In bacteria, two distinct G3P acyltransferases (GPATs), PlsB and PlsY, catalyse the committed step. By contrast, the recently identified membrane-integral PlsY exists exclusively and ubiquitously in bacteria, and uses an unusual acyl donor, namely the acyl-phosphate (acylP), representing a unique class of acyltransferase. PlsY acylates G3P using acylP, forming lysoPA and inorganic phosphate (Pi). The overall shape of aaPlsY resembles a funnel composed of three tilted helices (α1–3) sitting in a cup composed of seven TMHs.

Here we use X-ray crystallography to determine the PlsY structure at 1.48 Å resolution using crystals grown in an activity-supporting lipid bilayer environment, revealing a 7-TMH fold. By contrast, rod-shaped aaPlsY crystals were obtained in LCP made of 7.8 monoacylglycerol (MAG), a powerful host lipid for several crystallization projects. The structure (named as aaPlsYMAG) contains one complete aaPlsY monomer in each asymmetric unit. The striking shortness of TMH4 (n = 11) is compensated by the membrane-embedded Loop3. The overall structure is very compact; apart from two relatively long cytoplasmic loops containing functionally important residues, the helices are stitched together with short linkers. As noted, MAG resembles acylP and lysoPA; and indeed, the MAG molecule in the active site is almost superimposable with the lipid substrate and product. Thus, the collective poses of the MAG molecules near the gate are reminiscent of the snapshots for the exchange of acylP and lysoPA between the active site and the membrane. Despite the different states, the five structures are superimposable with root-mean-square deviation values within 0.52 Å, suggesting a lack of flexibility.

> MGSALFLVIFAYLLGSITFGEVIAKLKGVDLRNVGSGNVGATNVTRALGKKYGVLVFFLDFLKGFIPALIAVKSFGIDSWVLTFTGLASVLGHMYPVFFGFKGGKGVATALGVVFAVSPSVALFSFLVWLGIFLWKRYVSLASITATISAFLFLFVAGYPVNVLFMAIVIGALIIYRHRENINRLLTGREHRFGTLEVLFQ>MSQRITIDPVTRIEGHLRIDCEIENGVVSKAWASGTMWRGMEEIVKNRDPRDAWMIVQRICGVCTTTHALSSVRAAESALNIDVPVNAQYIRNIILAAHTTHDHIVHFYQLSALDWVDITSALQADPTKASEMLKGVSTWHLNSPEEFTKVQNKIKDLVASGQLGIFANGYWGHPAMKLPPEVNLIAVAHYLQALECQRDANRVVALLGGKTPHIQNLAVGGVANPINLDGLGVLNLERLMYIKSFIDKLSDFVEQVYKVDTAVIAAFYPEWLTRGKGAVNYLSVPEFPTDSKNGSFLFPGGYIENADLSSYRPITSHSDEYLIKGIQESAKHSWYKDEAPQAPWEGTTIPAYDGWSDDGKYSWVKSPTFYGKTVEVGPLANMLVKLAAGRESTQNKLNEIVAIYQKLTGNTLEVAQLHSTLGRIIGRTVHCCELQDILQNQYSALITNIGKGDHTTFVKPNIPATGEFKGVGFLEAPKGMLSHWMVIKDGIISNYQAVVPSTWNSGPRNFNDDVGPYEQSLVGTPVADPNKPLEVVRTIHSFDPCMACAVHVVDADGNEVVSVKVL[2x];>MAESVTNPQRPPVIWIGAQECTGCTESLLRATHPTVENLVLETISLEYHEVLSAAFGH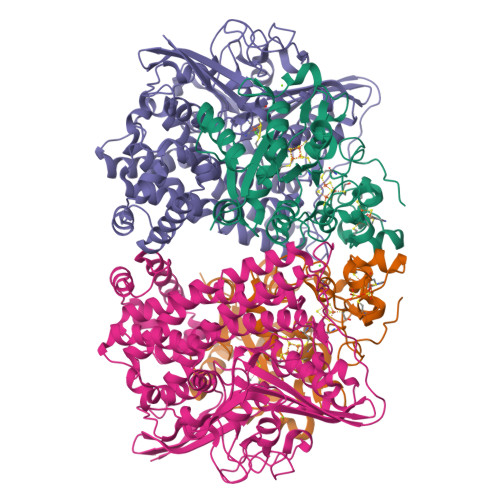QVEENKHNALEKYKGQYVLVVDGSIPLKDNGIYCMVAGEPIVDHIRKAAEGAAAIIAIGSCSAWGGVAAAGVNPTGAVSLQEVLPGKTVINIPGCPPNPHNFLATVAHIITYGKPPKLDDKNRPTFAYGRLIHEHCERRPHFDAGRFAKEFGDEGHREGWCLYHLGCKGPETYGNCSTLQFCDVGGVWPVAIGHPCYGCNEEGIGFHKGIHQLANVENQTPRSQKPDVNAKEGGHHHHHH[2x]>MSWLTEEDIRRWESGTFYDSYRKLGAHPDEEGTWFCVWAPHADAVSVLGAFNNWDPEAHQLERYGAGLWAGYVPGALPGHAYKYRIRHGFYQADKTDPYAFAMEPPTGSPIEGLASIITRLDYTWHDDAWMQRRKGPASLYEPVSIYEVHLGSWRHKQPGVSFSYREIAEPLADYVQDLGFTHVELLPIMEHPYYGSWGYQVVGYYAPTFRYGTPQDLMYLIDYLHQRGIGVILDWVPSHFAADPQGLVYFDGTTLFEYDDPRMRHHPDWGTYVFDYNKPGVRNFLISNALFWLDYYHVDGLRVDAVASMLYRDYSRKEWTPNIFGGRENLEAIDFIKKFNETVYLHFPEAITIAEESTAWPGVSAPTYNNGLGFLYKWNMGWMHDTLDYMRRDPVHRKYHHDTLTFSLWYAFSEHYILPLSHDEVVHGKGSLWTKMPGDDWQKAANLRLLYGHMWGH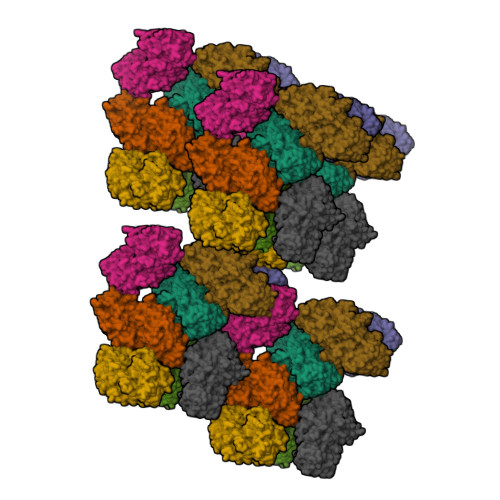PGKKLLFMGGEFGQHHEWNHDTQLEWHLLDQPYHRGIQAWVRDLNHLYRTHPALWHDGPEGFEWIDFNDRDQSVICYLRKHTDRLLLFVLNFTPVPREHYRVGVPIGGPWREVLNSDAVAYGGSGMGNFGRVEAVPESWHGRPFHLELTLPPLAILILEPES[8x]>[6x]MVLDLDLFRVDKGGDPALIRETQEKRFKDPGLVDQLVKADSEWRRCRFRADNLNKLKNLCSKTIGEKMKKKEPVGDDESVPENVLSFDDLTADALANLKVSQIKKVRLLIDEAILKCDAERIKLEAERFENLREIGNLLHPSVPISNDEDVDNKVERIWGDCTVRKKYSHVDLVVMVDGFEGEKGAVV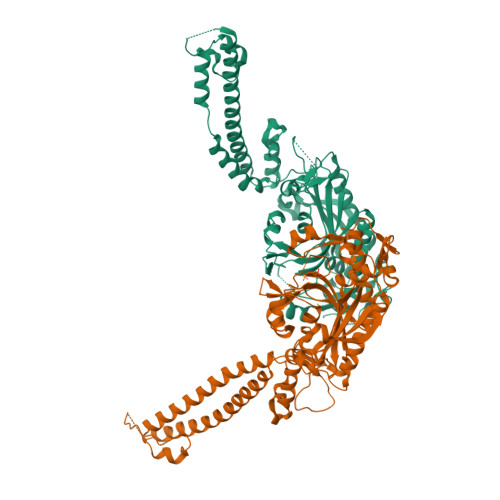AGSRGYFLKGVLVFLEQALIQYALRTLGSRGYIPIYTPFFMRKEVMQEVAQLSQFDEELYKVIGKGSEKSDDNSYDEKYLIATSEQPIAALHRDEWLRPEDLPIKYAGLSTCFRQEVGSHGRDTRGIFRVHQFEKIEQFVYSSPHDNKSWEMFEEMITTAEEFYQSLGIPYHIVNIVSGSLNHAASKKLDLEAWFPGSGAFRELVSCSNCTDYQARRLRIRYGQTKKMMDKVEFVHMLNATMCATTRTICAILENYQTEKGITVPEKLKEFMPPGLQELIPFVKPAPIEQEPSKKQKKQHEGSKKKAAARDVTLENRLQNMEVTDALEHHHHHH> QAMVTRCEPVVCYLYGKRGGGKSLTSIALATKICKHYGVEPEKNIYTKPVASDYWDGYSGQLVCIIDDIGQNTTDEDWSDFCQLVSGCPMRLNMASLEEKGRHFSSPFIIATSNWSNPSPKTVYVKEAIDRRLHFKVEVKPASFFKNPHNDMLNVNLAKTNDAIKDMSCVDLIMDGHNVSLMDLLSSLV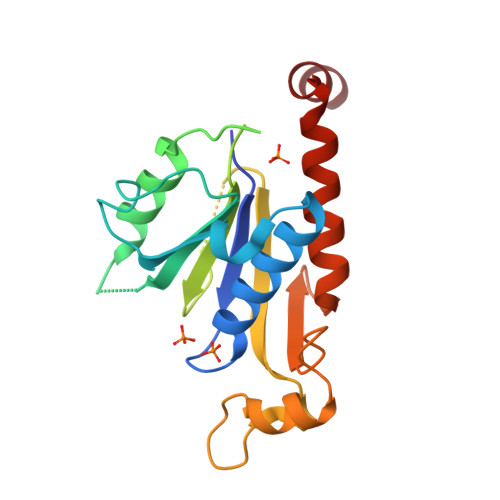MTVEIRKQNMTEFMELWSQ> MSQRITIDPVTRIEGHLRIDCEIENGVVSKAWASGTMWRGMEEIVKNRDPRDAWMIVQRICGVCTTT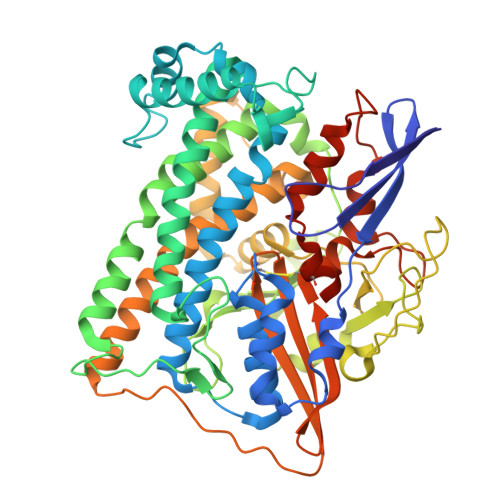HALSSVRAAESALNIDVPVNAQYIRNIILAAHTTHDHIVHFYQLSALDWVDITSALQADPTKASEMLKGVSTWHLNSPEEFTKVQNKIKDLVASGQLGIFANGYWGHPAMKLPPEVNLIAVAHYLQALECQRDANRVVALLGGKTPHIQNLAVGGVANPINLDGLGVLNLERLMYIKSFIDKLSDFVEQVYKVDTAVIAAFYPEWLTRGKGAVNYLSVPEFPTDSKNGSFLFPGGYIENADLSSYRPITSHSDEYLIKGIQESAKHSWYKDEAPQAPWEGTTIPAYDGWSDDGKYSWVKSPTFYGKTVEVGPLANMLVKLAAGRESTQNKLNEIVAIYQKLTGNTLEVAQLHSTLGRIIGRTVHCCELQDILQNQYSALITNIGKGDHTTFVKPNIPATGEFKGVGFLEAPKGMLSHWMVIKDGIISNYQAVVPSTWNSGPRNFNDDVGPYEQSLVGTPVADPNKPLEVVRTIHSFDPCMACAVHVVDADGNEVVSVKVL(2S)-1-(2,5-dimethylphenoxy)-3-morpholin-4-ylpropan-2-ol 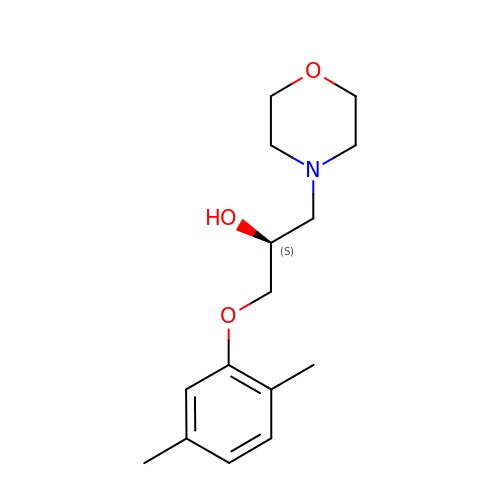| C15 H23 N O3 | HVMGGHDPXHODHE-AWEZNQCLSA-N>[2x]MSVLNTPNHYKMDNSGRRVVIDPVTRIEGHMRCEVNVDENNVIQNAVSTGTMWRGLEVILRGRDPRDAWAFVERICGVCTGCHALASVRAVEDALDIKIPHNATLIREIMAKTLQIHDHIVHFYHLHALDWVNPVNALKADPQATSELQKLVSPHHPMSSPGYFKDIQIRIQKFVDSGQLGIFKNGYWSNPAYKLSPEADLMAVTHYLEALDFQKEIVKIHAIFGGKNPHPNYMVGGVPCAINIDGDMAAGAPINMERLNFVKSLIEQGRTFNTNVYVPDVIAIAAFYRDWLYGGGLSATNVMDYGAYPKTPYDKSTDQLPGGAIINGDWGKIHPVDPRDPEQVQEFVTHSWYKYPDETKGLHPWDGITEPNYELGSKTKGSRTNIIEIDESAKYSWIKSPRWRGHAVEVGPLARYILAYAQG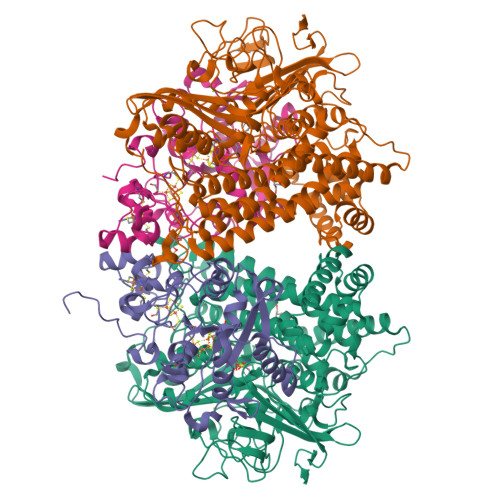VEYVKTQVHTSLNRFNAVCRLLDPNHKDITDLKAFLGSTIGRTLARALESEYCGDMMLDDFNQLISNIKNGDSSTANTDKWDPSSWPEHAKGVGTVAAPRGALAHWIVIEKGKIKNYQCVVPTTWNGSPRDPKGNIGAFEASLMGTPMERPDEPVEVLRTLHSFDPCLACSTH;>NKIAHAMETKPRTPVIWLHGLECTCCSESFIRSAHPLAKDVVLSMISLDYDDTLMAASGHAAEAILDEIKEKYKGNYILAVEGNPPLNQDGMSCIIGGRPFSEQLKRMADDAKAIISWGSCASWGCVQAAKPNPTQATPVHKFLGGGYDKPIIKVPGCPPIAEVMTGVITYMLTFDRIPELDRQGRPKMFYSQRIHDKCYRRPHFDAGQFVEEWDDEGARKGYCLYKVGCKGPTTYNACSTVRWNGGTSFPIQSGHGCIGCSEDGFWDKGSFYSRDTEMNAFG[2x]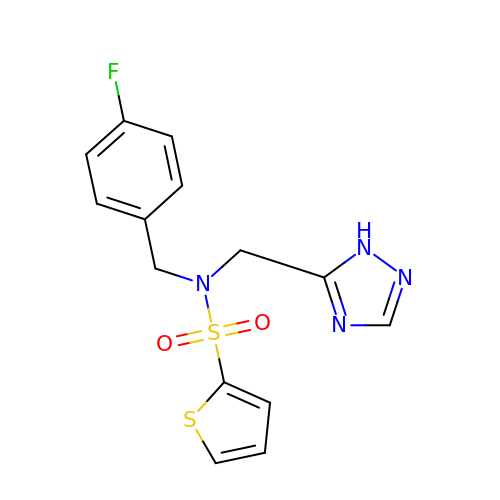~{N}-[(4-fluorophenyl)methyl]-~{N}-(1~{H}-1,2,4-triazol-5-ylmethyl)thiophene-2-sulfonamide | C14 H13 F N4 O2 S2 | UGVZRLMKBSBNEC-UHFFFAOYSA-N>GAMAGVFTYETEFTSVIPPPRLFKAFILDADNLIPKIAPQAVKCAEIIEGDGGVGTIKKITFGEGSQFGSVTHKIDGIDKENFVYSYSLIEGDALSDKIEKISYETKLVSSSDGGSIIKSTSNYHTKGDVEIKEEHVKAGKEKASHLFKL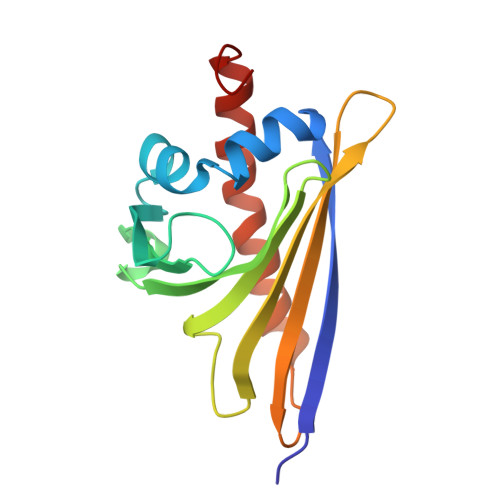VEGYLLANPNEYC[2x]alpha-L-sorbopyranose | C6 H12 O6 | 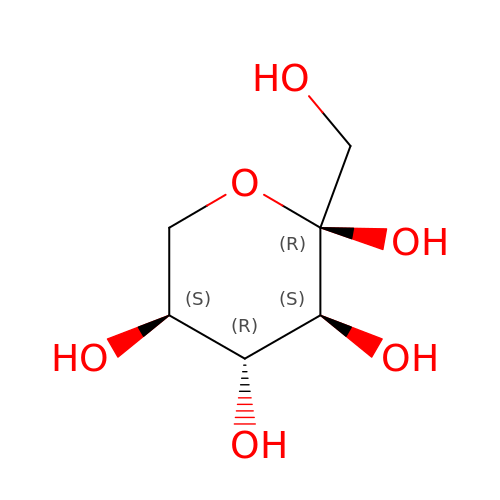LKDRXBCSQODPBY-BGPJRJDNSA-N2',3'-DIDEOXYCYTOSINE-5'-DIPHOSPHATE | C9 H15 N3 O9 P2 | 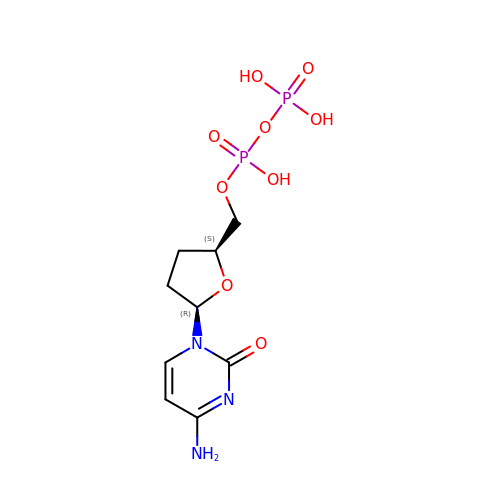FVSQWXITYSICAK-POYBYMJQSA-N The NADPH-dependent FAD-containing oxidoreductase mycothiol disulfide reductase (Mtr) is known to reduce oxidized mycothiol disulfide (MSSM) to MSH, which is crucial to maintain the cellular redox balance. Mtr belongs to a group of NAD(P)H-dependent homodimeric oxidoreductases with a tightly bound flavin adenine dinucleotide (FAD) cofactor per subunit. The crystal structures of Mtr Re and Mtr Ms confirm that Mtr is a homodimer, as also supported by molecular-weight estimations during protein purification. Each monomer, composed of 458 and 461 residues in Mtr Re and Mtr Ms , respectively, belongs to the pyridine nucleotide-disulfide oxidoreductase (PNDO) superfamily and consists of three domains, namely a NAD(P)H-binding domain, a FAD-binding domain and a dimerization/interface domain. In addition, each subunit contains a catalytic redox-active disulfide/Cys pair that is responsible for the reduction of their respective and structurally unique disulfide-bonded substrates.

Two structures of Mtrs from homologous Actinobacteria are presented in this work; Mtr Ms from the M. tuberculosis model organism M. smegmatis and Mtr Re from R. erythropolis, a biocatalyst used for the bioremediation of toxic compounds. In addition, a strongly comparable A 465 nm/A 280 nm ratio for both proteins, as well as the yellow crystals obtained of Mtr Re and Mtr Ms , support the presence of FAD in both proteins, although FAD could not be built into the Mtr Ms structure due to its low resolution and lack of significant density. Together, these results demonstrate that the detailed structural features observed and described for the structure of Mtr Re are representative of both Mtr Re and Mtr Ms , as well as other Mtrs across species. In contrast to the previously reported asymmetric SAXS structure of Mtr, the crystallographic Mtr structures from M. smegmatis and R. erythropolis presented in this work display a symmetrical topology, as described for most homologous oxidoreductase structures.

>[2x]MEHYDLAIIGTGSGNSIVDDRYAGKKVAICEQGTFGGTCLNVGCIPTKMFVYAAEVAHSVRTSARYGVDAHIDKVRWPDIVERVFGRIDPIAAGGEDYRRSDPNITVYSSHTRFGPKTDDGRYTLRTESGEEFTSDQVVIAAGSRTYIPPAVVDCGVKYHTSDDIMRIPELPTDLVIIGGGFVSAEFAHVFSALGVHVTIVVRGDGLLTHCDETICHRFNEIAATKWDIRTHENVIGSHQDGDRIVLELDDGKTVAADTLLVATGRVPNGDLLDAELAGVEVDEDGRVIVDQYQRTTARGVFALGDVSSDYQLKHVANHEARVVKENLLRDWDDTASLVASDHRFVPSAVFTDPQVATVGLTEAEARAAGHDIVVKVQNYGDTAYGWAMEDTTGIAKLIGERGTGKLLGAHILGHQASSIIQPLIQAMSLGQTAQEIARGQYWIHPALPEVIENALLGLQE> ISEFGSSHSTNDAKSPTLSESHKSARNVLENIGIKIYNQEIKKKNPYEQQLKGTLSRAQFVDALSSRYGYVRNSDGNSCNLDHLFHTNIKTGYNEGRKPCYGREQNRFDENAEAYCNSDKIRGNENNANGAACAPPRRRHICDQNLEFLDNKNTNTAHDLLGNVLVTAKYEGNYIVNDHPDKNSNGNKAGICTSLARSFADIGDIVRGRDMFLPNKDDKVQKGLQVVFKKIYKSLTPEARKHYAHGDGSGNYAKLREDWWTINREQIWKALTCSAPYYADYFRKGSDGTLHFSSHGKCGHNEGAPPTYLDYVPQFLRWFEEWSEEFCRIKKIKIDKVKKECRDEQNKKYCSGDGHDCTQTNLAHNQIFVDLDCPRCQDQCIKYNEWIVKKLEEFYKQNLKYSMEIQKWKKTKNNYYDKEFYENLDKKSYSTIDKFLNLLNNGKHCHDNKDEKNKIDFNKPIKTFSISEYCKTCPLYGVTCTNRGICIHNSNNKNKGENDLNKINIKDKSPTTFDVDMIYLRRQYMKNELKSFVESTCLFKGMRNQEWTCQILKNLDVCKLNNFNKVIDIDKHITFKVLLERWLKDFLEGYKKSKRKINPCTKDKNSCIKLCINKCTCVEEWLNKKEKEWGQIKKHFNKQFHGEG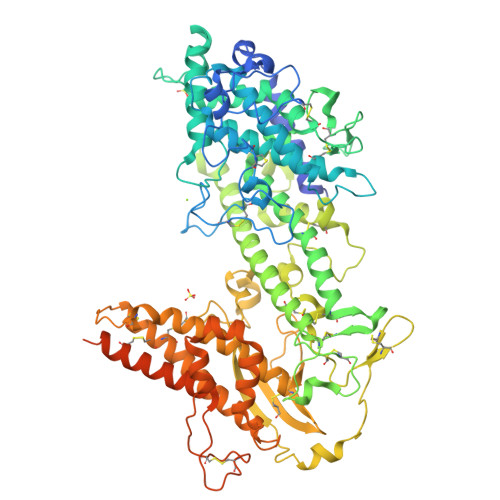YDIAFKVKSYFEDNEADVRKSIDNFHVLKNKEEYEICNVDDNCRSQNNKKKKDIVTILLKELKDKIVSCKNQHKATKGKECCDKLPKIADGDTSDDEEQEDEAPAPPKPKPPSTPNPCVRKDQSGTHIVSVEDVAEWMQGVTHDRV> MCSSINEGPYNSPTFGKSLSLKVDGGFNAVSINPSGRDIVLASRQGLYIIDLDDPFTPPRWLHHITPWQVADVQWSPHPAKPYWIVSTSNQKAIIWNLAKSSSNAIEFVLHGHSRAITDINFNPQHPDVLATCSVDTYVHAWDMRSPHRPFYSTSSWRSAASQVKWNYKDPNVLASSHGNDIFVWDLRKGSTPLCSLKGHVSSVNSIDFNRFKYSEIMSSSNDGTVKFWDYSKSTTESKRTVTTNFPIWRGRYLPFGEGYCIMPMVGGNNAVYLINLCDDDDSEQNKKTKLQPIYAFKGHSDRVIDFLWRSRHTCDGDYDDREFQLVTWSKDCDLKLWPISDSIYGKVNFDRGKRLEEKLPDYDYCSYNKEPENRENVQKNEFRRLRENFVTTSGLKKNKTNHITWLSGIRMNSATSQEDLFNETK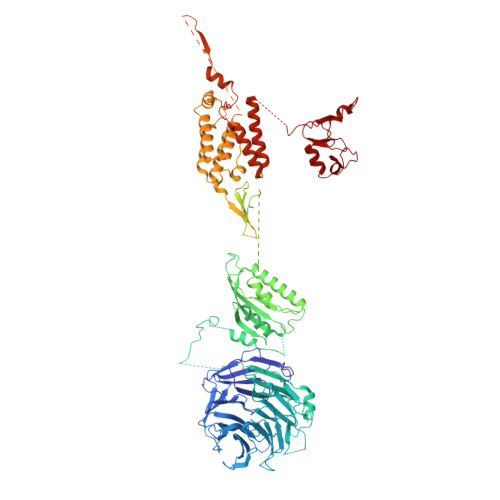IQNLGEEVSAIGHKFPKVVFEKISVSTRELCLTLNGPWSEENPDDYIFLRISINFPLNYPNKGDPPKFTIEENSNLTMSKRQEILSNLATIGQKYTDSNLYCLEPCIRFVLGEKVSLEDIEEGQEPLLNFDIADHIDFEELSSLDSSYSDSQNPENLSSQSDIESYKEALVFPDTSNQGLDFGRNLALDTTPVPNGCGSCWTATGELFCFFANEKKPEKKQNAIIKLSQKEAGVEKHPFKIEPQVLYDKEVDSSVITAADELKARPKRYVDTLGLGGGTNGDSRTYFDDETSSDDSFDSVADDWDDILRNDIIVRTKIPILRGNFKAFSSVHSESGKTVESTKKNKNLVISKNFSSLLSDRKELALEYLFMDATPEGFARNNALVAEKFDLDEISHCWQILSDMLIDQSDYDPYTTIWNNHPMGIKWFIKEAIVYFERQQNLQMLAMLCCVILSARRKKIPARYYGQELENMEGTIVFNDNESQNTSFWKGSDAFSTRSRSSTVTPNFYGNHLRGKNIHGGDNSSIRSDDHHARLRTHNTLNGSSKFTEPAQKQGSRAISSSPFHSRMPDIKVELLHDDIIEAYEQEDLLHLEVSDIPKFQTYIYQYSKLLFRWGLPLERVKILKVSTDFRSSYSSQGIPPNNNKKSPYNGVLTHWIENNEFGEEKFLARNCNYCDLRVTRSSFICGNCQHVLHSSCARIWWEIGDECPSGCGCNCPEMFDA> MVKPNWDNFKAKFSENPQGNFEWFCYLLFCQEFKMPAGIFRYKNQSGIETNPITKDNEIIGWQSKFYDTKLSDNKADLIEMIEKSKKAYPGLSKIIFYTNQEWGQGRKSHEPEGDKNADNYLETVGNSNDPKIKIEVDQKAYESGIEIVWRVASFFESPFVIVENEKIAKHFFSLNESIFDLLEEKRKHTENVLYEIQTNIEFK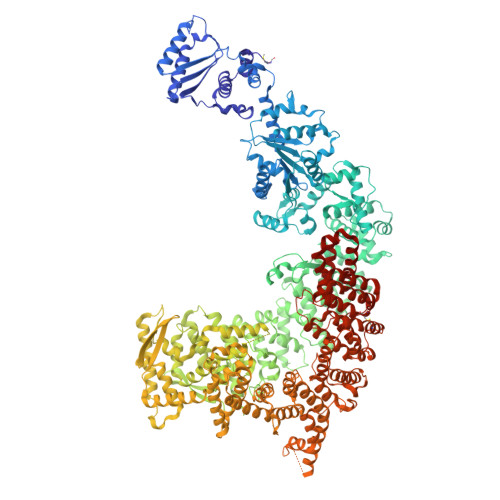DRSIEIDRRHCIELLHENLVQKKIVIVSGEGGVGKTAVIKKIYEAEKQYTPFYVFKASEFKKDSINELFGAHGLDDFSNAHQDELRKVIVVDSAEKLLELTNIDPFKEFLTVLIKDKWQVVFTTRNNYLADLNYAFIDIYKITPGNLVIKNLERGELIELSDNNGFSLPQDVRLLELIKNPFYLSEYLRFYTGESIDYVSFKEKLWNKIIVKNKPSREQCFLATAFQRASEGQFFVSPACDTGILDELVKDGIVGYEAAGYFITHDIYEEWALEKKISVDYIRKANNNEFFEKIGESLPVRRSFRNWISERLLLDDQSIKPFIAEIVCGEGISNFWKDELWVAVLLSDNSSIFFNYFKRYLLSSDQNLLKRLTFLLRLACKDVDYDLLKQLGVSNSDLLSIKYVLTKPKGTGWQSVIQFIYENLDEIGIRNINFILPVIQEWNQRNKVGETTRLSSLIALKYYQWTIDEDVYLSGRDNEKNILHTILHGAAMIKPEMEEVLVKVLKNRWKEHGTPYFDLMTLILTDLDSYPVWASLPEYVLQLADLFWYRPLKETGERYHSMDIEDEFGLFRSHHDYYPESPYQTPIYWLLQSQFKKTIDFILDFTNKTTICFAHSHFAKNEIEEVDVFIEEGKFIKQYICNRLWCSYRGTQVSTYLLSSIHMALEKFFLENFKNADSKVLESWLLFLLRNTKSASISAVVTSIVLAFPEKTFNVAKVLFQTKDFFRFDMNRMVLDRTHKSSLISLRDGFGGTDYRNSLHEEDRIKACDDVHRNTYLENLALHYQIFRSENVTEKDAIERQQVLWDIFDKYYNQLPDEAQETEADKTWRLCLARMDRRKMKITTKEKDEGIEISFNPEIDPKLKQYSEEAIKKNSEHMKYVTLKLWASYKREKDERYKNYGMYEDNPQIALQETKEIIKKLNEEGGEDFRLLNGNIPADVCSVLLLDYFNQLNNEEREYCKDIVLAYSKLPLKEGYNYQVQDGTTSAISALPVIYHNYPMERETIKTILLLTLFNDHSIGMAGGRYSVFPSMVIHKLWLDYFDDMQSLLFGFLILKPKYVILSRKIIHESYRQVDYDIKKININKVFLNNYKHCISNVIDNKISIDDLGSMDKVDLHILNTAFQLIPVDTVNIEHKKLVSLIVKRFSTSLLSSVREDRVDYALRQSFLERFAYFTLHAPVSDIPDYIKPFLDGFNGSEPISELFKKFILVEDRLNTYAKFWKVWDLFFDKVVTLCKDGDRYWYVDKIIKSYLFAESPWKENSNGWHTFKDSNSQFFCDVSRTMGHCPSTLYSLAKSLNNIASCYLNQGITWLSEILSVNKKLWEKKLENDTVYYLECLVRRYINNERERIRRTKQLKQEVLVILDFLVEKGSVVGYMSRENIL>GPMAVPFSNTHLRIPRGFGNLLEGLTREVLREQPEDIATFAAVYFTELLKAREESGLDPAEWGAKLEDRFYNNH[4x]

By combining bioinformatic and phylogenetic analyses with structural approaches, we have discovered that the docking and dimerization (D/D) domain of the PKA regulatory subunit is an ancient and conserved protein fold. An archetypal function of this module is to interact with A-kinase-anchoring proteins (AKAPs) that facilitate compartmentalization of this key cell-signaling enzyme. The sperm autoantigenic protein 17 (SPA17) is a prototype of the type II or R2D2 subgroup that is conserved across metazoan phyla. In solution, SPA17 forms both homodimers and tetramers and displays a weak affinity for AKAP18.

A construct spanning amino acids 1 to 75 of SPA17 from D. rerio was expressed in Escherichia coli, and the resultant protein was purified with a sequential three-step affinity, anion-exchange, and size-exclusion chromatography (SEC) protocol. Crystals of SPA17 diffracted X-ray to 1.72 Å. Four copies of SPA17 are observed in the asymmetric unit of the crystal. The two central copies of SPA17 form the canonical four-helix bundle as previously observed in the homodimeric D/D domains of R1 and RII. Interestingly, the two conserved sequence regions flanking the central helices of SPA17 both adopt a regular β-strand conformation. A four-stranded β-sheet is formed from the amino-terminal β-strand of two SPA17 molecules and the carboxyl-terminal β-strands of two other SPA17 chains. Alignment of the SPA17 structure to the D/D domain of apo RIIα dimers results in an associated RMSD of 0.482 Å. The AKAP-binding site is, therefore, retained in the SPA17 homodimer, although it appears to be occluded by the β-sheet formed among the terminal strands of SPA17 protomers in the crystal. SEC coupled to multiangle light scattering (SEC-MALS) verifies that SPA17 tetramers and dimers exist in solution. Homomeric SPA17 bound AKAP18 with an affinity of 9.6 ± 0.69 μM, supporting the notion that its AKAP-binding site is not blocked by the terminal β strands.>[6x]MALAKRIDAALIVKDGRVVKGSNFENLRDSGDPVELGKFYSEIGIDELSFWDITASVEKRKTMLELVEKVAEQIDIPFTVGGGIHDFETASELILRGADKVEINTAAVENPSLITQIAQTFGSQAVVVYIAAKRVDGEFMVF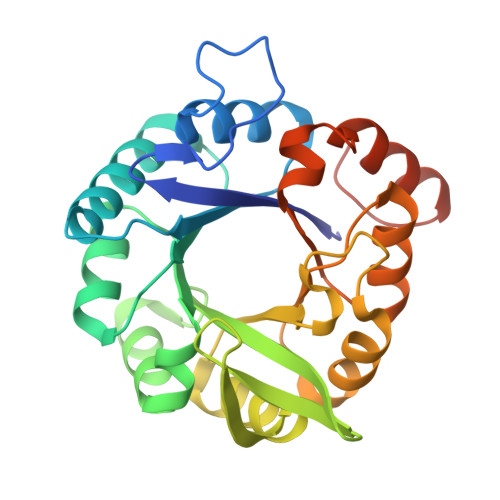TYSGEKNTGILLRDWVVEVEKRGAGEIVLGSIDRLGTKSGYDTEMIRFVRPLTTLPIIAHRGAGKMEHFLEAFLAGADAAKADSVFHFREIDVRELKEYLKKHGVNVRLEGLGSHHHHHH>KHMKEIVFGTTVGDFGDMVKEQIQAELEKKGYTVKLVEFTDYVRPNLALAEGELDINVFQHKPYLDDFKKEHNLDITEVFQVPTAPLGLYPGKLKSLEEVKDGSTVSAPNDPSNFARVLVMLDELGWIKLKDGINPLTASKADIAENLKNIKIVELEAA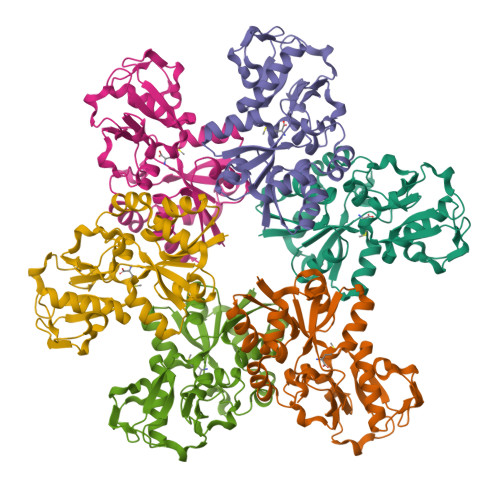QLPRSRADVDFAVVNGNYAISSGMKLTEALFQEPSFAYVNWSAVKTADKDSQWLKDVTEAYNSDAFKAYAHKRFEGYKSPAAWNEGAAK[6x]> MAPVHVDNPYAGAVQYVNPTWAASVNAAAGRQSADPALAAKMRTVAGQPTAVWMDRISAITGNADGNGLKFHLDNAVAQQKAAGVPLVFNLVIYDLPGRDCFALASNGELPATDA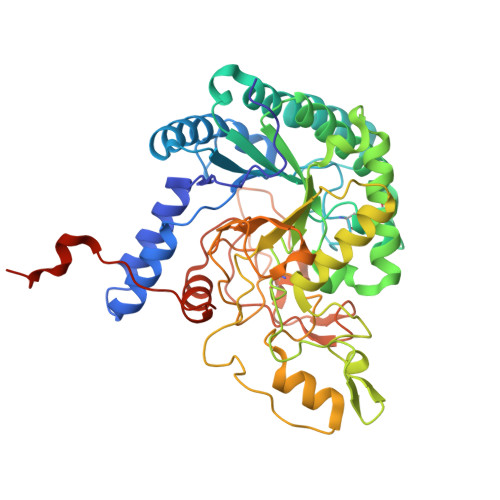GLARYKSEYIDPIADLLDNPEYESIRIAATIEPDSLPNLTTNISEPACQQAAPYYRQGVKYALDKLHAIPNVYNYIDIGHSGWLGWDSNAGPSATLFAEVAKSTTAGFASIDGFVSDVANTTPLEEPLLSDSSLTINNTPIRSSKFYEWNFDFDEIDYTAHMHRLLVAAGFPSSIGMLVDTSRNGWGGPNRPTSITASTDVNAYVDANRVDRRVHRGAWCNPLGAGIGRFPEATPSGYAASHLDAFVWIKPPGESDGASTDIPNDQGKRFDRMCDPTFVSPKLNNQLTGATPNAPLAGQWFEEQFVTLVKNAYPVIGGTTPVEDLVAPTIEGRFGGHHHHHH>[2x]ETAIPFSRRRMPYSLGTDKLEKVDPDKIKSKLSEDVERKLETDMRELYDRLLPT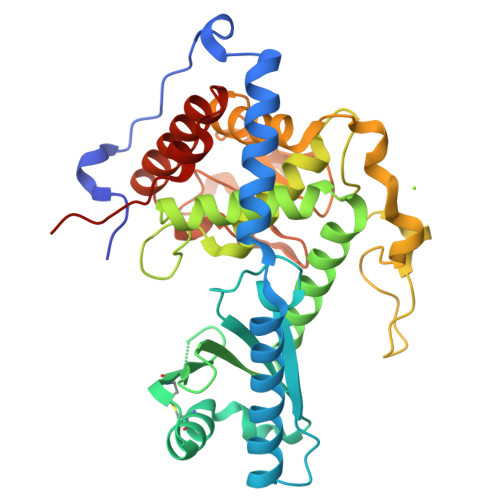EAIEVNRRELVSKLERLFNTEWPGHDIRVHLFGSSGNLLCSDDSDVDICITTPWRELESVCMIAELLDRHGMEKVVCVSSAKVPIVKIWDPELKLACDMNVNNTLALENTRMVRTYVSIDDRVRPLAMIIKYWTRRRVVNDAAFGGTLSSYTWICMIIAFLQLRDPPVLPALHQQHDLKLVKQDGALSDFADDIPKLRGFGAKNKDSLAVLLFQFFRFYAHEFDYDKYTLSIRMGTLLTKAEKNWQYLVNNALCVEEPFNDGRNLGNTADETSFRGLHMELRRAFDLIAEGKLEECCEQYVFPKEEERV(6-butoxy-1-benzofuran-3-yl)acetic 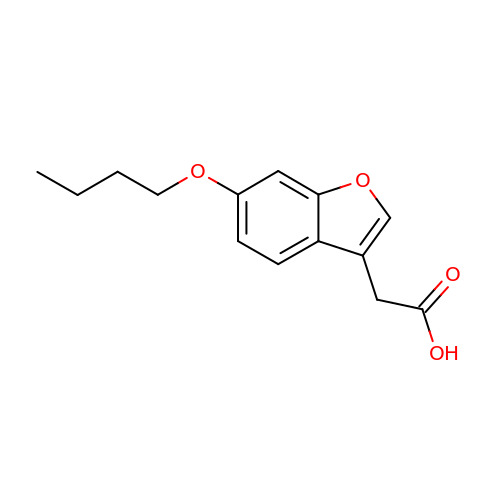acid | C14 H16 O4 | SZOTYOZQWWESFH-UHFFFAOYSA-N>SNAMTHETDQLYQAVQATRPLLRNITAAVERGTLREGVTVGQRAILEGLSLTPGATAPQLGAALQMKRQYISRILQEVQRAGLIERRTNPEHARSHRYWLTPRGEAIITAIRAD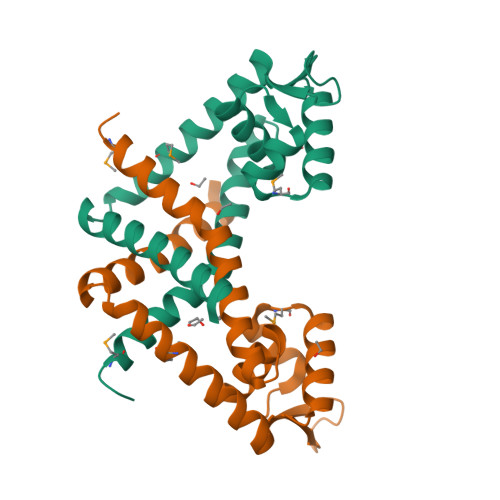EMAKLALFSEGFSSVELTAYHKVQLALTRFFADLAKEA[2x]>[2x]QLTIEVLVTVDGVNFRTV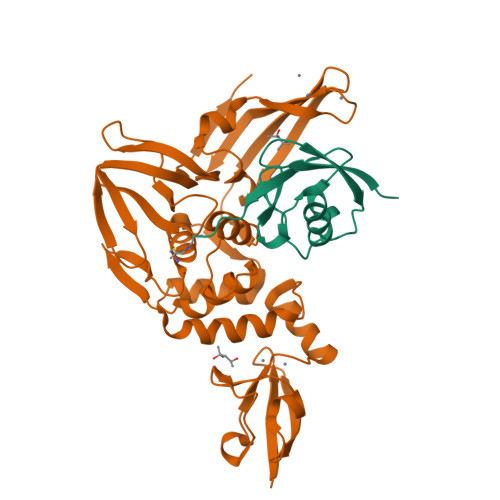VLNNKNTYRSQLGCVFFNGADISDTIPDEKQNGHSLYLADNLTADETKALKELYGPVDPTFLHRFYSLKAAVHGWKMVVCDKVRSLKLSDNNCYLNAVIMTLDLLKDIKFVIPALQHAFMKHKGGDSTDFIALIMAYGNCTFGAPDDASRLLHTVLAKAELCCSARMVWREWCNVCGIKDVVLQGLKACCYVGVQTVEDLRARMTYVCQCGGERHRQLVEHTTPWLLLSGTPNEKLVTTSTAPDFVAFNVFQGIETAVGHYVHARLKGGLILKFDSGTVSKTSDWKCKVTDVLFPGQKYSSDCN;>[2x]MEPLSILVRNNKGRSSTYEVRLTQTVAHLKQQVSGLEGVQDDLFWLTFEGKPLEDQLPLGEYGLKPLSTVFMNLRLRG7-Chlorokynurenic acid | C10 H6 Cl N O3 | 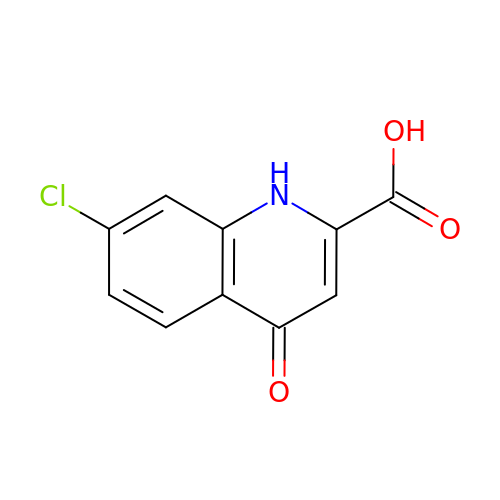UAWVRVFHMOSAPU-UHFFFAOYSA-N> EVKQENRLLNESESSSQGLLGYYFSDLNFQAPMVVTSSTTGDLSIPSSELENIPSENQYFQSAIWSGFIKVKKSDEYTFATSADNHVTMWVDDQEVINKASNSNKIRLEKGRLYQIKIQYQRENPTEKGLDFKLYWTDSQNKKEVISSDNLQLPELKQK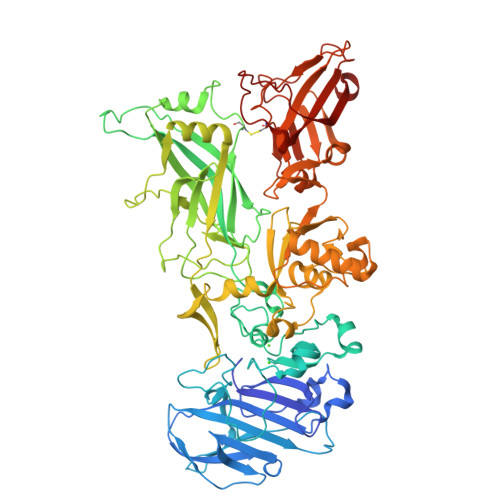SSNSRKKRSTSAGPTVPDRDNDGIPDSLEVEGYTVDVKNKRTFLSPWISNIHEKKGLTKYKSSPEKWSTASDPYSDFEKVTGRIDKNVSPEARHPLVAAYPIVHVDMENIILSKNEDQSTQNTDSQTRTISKNTSTSRTHTSEPGSNSNSSTVAIDHCLSLAGERTWAETMGLNTADTARLNANIRYVNTGTAPIYNVLPTTSLVLGKNQTLATIKAKENQLSQILAPNNYYPSKNLAPIALNAQDDFSSTPITMNYNQFLELEKTKQLRLDTDQVYGNIATYNFENGRVRVDTGSNWSEVLPQIQETTARIIFNGKDLNLVERRIAAVNPSDPLETTKPDMTLKEALKIAFGFNEPNGNLQYQGKDITEFDFNFDQQTSQNIKNQLAELNATNIYTVLDKIKLNAKMNILIRDKRFHYDRNNIAVGADESVVKEAHREVINSSTEGLLLNIDKDIRKILSGYIVEIEDTEGLKEVINDRYDMLCISSLRQDGKTFIDFKKYNDKLPLYISNPNYKVNVYAVTKENTIINPSENGDTSTNGIKKILIFSKKGYEIG>MASKGNVDLVFLFDGSMSLQPDEFQKILDFMKDVMKKLSNTSYQFAAVQFSTSYKTEFDFSDYVKWKDPDALLKHVKHMLLLTNTFGAINYVATEVFREELGARPDATKVLIIITDGEATDSGNIDAAKDIIRYIIGIGKHFQTKESQETLHKFASKPASEFVKILDTF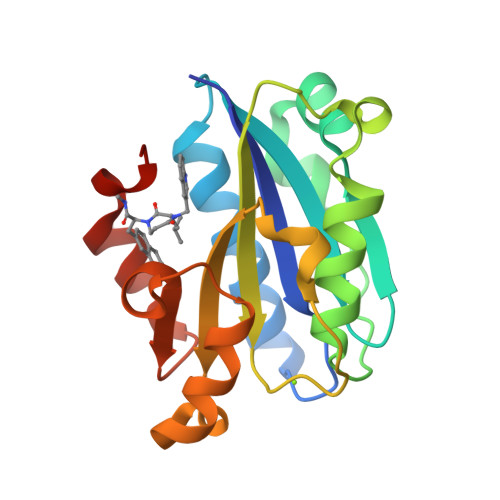EKLKDLFTELQKKIYVIEG[2x]>MAHHHHHHVGTFENITAAPADPILGLADLFRADERPGKVDLGVGVYKDETGKTPVLTSVKKAEQYLLENETTKTYLGLDGLPEFGRCTQELLF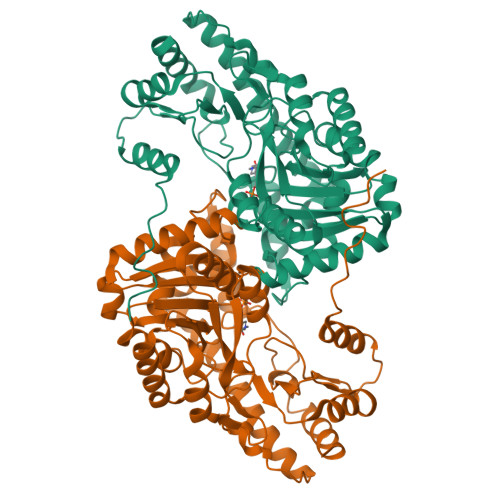GKGSALINDKRARTAQTPGGSGALRVGADFLAKNTSVKRVWVSNPSWPNHKAIFNSAGLEVREYAYYDAENHTLDFDALINSLNEAQAGDVVLFHGCCHNPTGIDPTLEQWQTLAQLSVEKGWLPLIDFAYQGFGRGLEEDAEGLRAFAAMHKELIVASSYSKNFGLYNERVGACTLVAADSETVDRAFSQMKAAIRANYSNPPAHGASVVATILSNDALRAIWEQELTDMRQRIQRMRQLFVNTLQEKGANRDFSFIIKQNGMFSFSGLTKEQVLRLREEFGVYAVASGRINVAGMTPDNMAPLCEAIVAVL[2x]> SMSDPVSYTRKDSIAVISMDDGKVNALGPAMQQALNAAIDNADRDDVGALVITGNGRVFSGGFDLKILTSGEVQPAIDM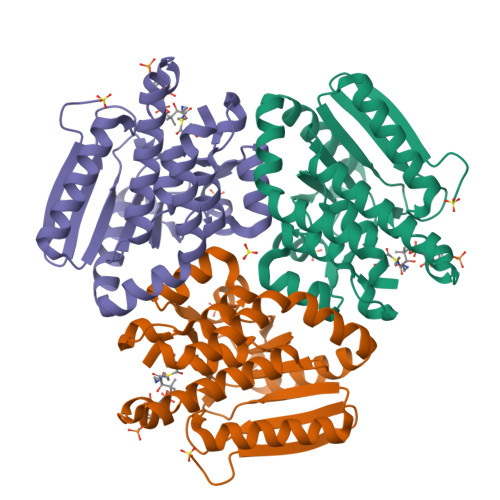LRGGFELAYRLLSYPKPVVMACTGHAIAMGAFLLSCGDHRVAAHAYNIQANEVAIGMTIPYAALEIMKLRLTRSAYQQATGLAKTFFGETALAAGFIDEIALPEVVVSRAEEAAREFAGLNQHAHAATKLRSRADALTAIRAGIDGIAAEFGL> MFENITTAPADPILGLADLLRADERPGKIDLGMGVYNDETGKTPVLTSVKKAEQYLLENETTKNYLGIDGIPEFGRCTQELLFGKGSALINDKRARTAQTPGGTGALRVAADFLAKNTSVRRVWVSNPSWPNHKSVFNSAGLEVREY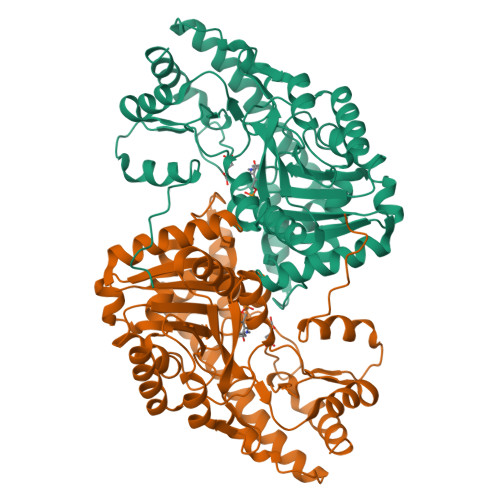AYYDAENHTLDFDALINSLNEAQAGDVVLFHGCCHNPTGIDPTLEQWQTLAQLSVEKGWLPLFDFAYQGFARGLEEDAEGLRAFAAMHKELIVASSYSKNFGLYNERVGTCTLVAADSETVDRAFSQMKAAIRVNYSSPPAHGASVVATILGNDALRAIWEQELTDMRQRIQRMRQLFVNTLQEKGANRDFSFTIKQNGMFFFGGLTKEQVLRLREEFGVYAVASGRLNVAGMTPDNLAPLCEAIVAVL>AGAGAGAGAGMKAILQLILEKRQEFEKLPCFEFVRDETISPEERLILYPCIAAFALNFRDLNRYDYRDDNSSDYYQKIINIHTQEDAKHWEWFLNDLELLGFDKTMRFSEALRFVWSDDLLHTRRLCHNIAVLSHDLEPVMKMVVIEAMETAGLVIFHALAKPGESIAKATRRKYLYVADSHVEVETGHAVGTENIITILEQTQLSSEQEEKAKEIVNKVFQWSTNLIGEFERYVKAHRSEKAQPTAAY[2x]

The biosynthesis of neurotoxin aetokthonotoxin (AETX) that features a unique structure of pentabrominated biindole nitrile involves a first-of-its-kind nitrile synthase termed AetD, an enzyme that shares very low sequence identity to known structures and catalyzes an unprecedented mechanism. AetD adopts the heme oxygenase like fold and forms a hydrophobic cavity within a helical bundle to accommodate the indole moiety. A diiron cluster comprising two irons that serves as a catalytic center binds to the carboxyl O and the amino N of the substrate. Akak et al. conducted biochemical analyses and confirmed that Fe(II) is required for AetD activity and the nitrogen atom in the nitrile is sourced from the α-amino group of the substrate instead of exogenous nitrogen or the enzyme residue.

Nonetheless, we successfully solved the structure of AetD/1 crystal that was not soaked with Fe ion. The AetD/1 structure harbors the substrate and a metal ion that is coordinated and located as the Fe1 observed in AetD/1/Fe. Based on the fact that the purified AetD carries Fe ion and the highly identical coordination status to other HO-like proteins, this metal ion should be reliably modeled with a Fe ion. Intriguingly, the Fe2-corresponding site is vacant and the Fe2-coordination networks are dissociated owing to the disordered helix α6 that deviates H179 away from the Fe2 site. Because AetD/1 and AetD/1/Fe share the same unit cell and space group, the conformational change of helix α6 is not a result of alternative crystal packing. Instead, it is possible that Fe ion in the soaking trial could bind to the enzyme and stabilize H179 to constitute the intact diiron cluster. Notably, a metal ion that is located distant from the Fe2 site and coordinated by waters, a TRIS and/or residues including E140 and H72 was observed in AetD/1. This metal was modeled with a Ni ion, whose presence could be competed by soaking crystals with Fe ion.> MAGLYTTYQLLEVQRKLKTLPAFFLQWFPRQINFQEDMIAFDKVIQDVTRVAPFVAP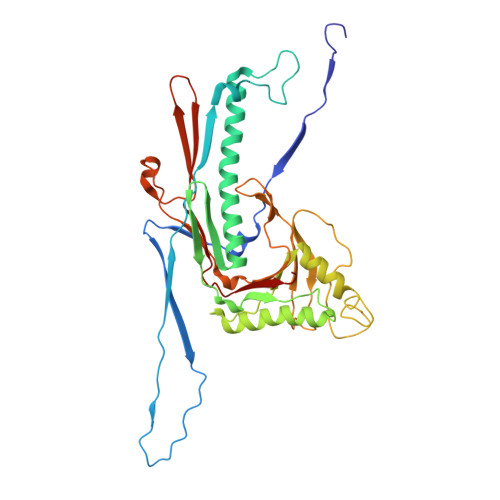NVQGRVIKESGYNTKTFKPAYVKPKHVIDPNMIIPRQPGEALGTGTLSIAQRRDRVIAYLLMKHRAMHENTWEWMAAQAAQYGYVDVQGQDYPLVRVDFGRDAALTMTTDWTAAGVTLMDMIADLRDGQRLVSDKSMSGTVIRDYIFGGDAWDQFVKVGGKELWGKDGLMDSTIRGSETNVTRLWDDVEGVQYMGELVGANGAGRMRIWVNTQKYRDQNDQEQFLMKQKAVMGISSAIEGVRCFGAILDKGAGYQALDYFPKMWDQEDPSVEYLMSQGAPLMVPADPNASFLLTVMS> MLNQELELSLNMAFARAREHRHEFMTVEHLLLALLSNPSAREALEACSVDLVALRQELEAFIEQTTPVLPASEEERDTQPTLSFQRVLQRAVFHVQSSGRNE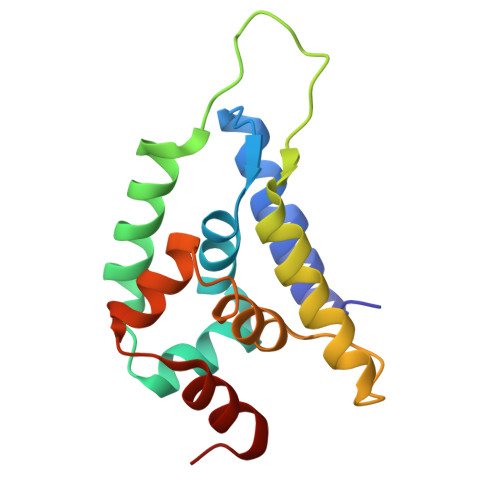VTGANVLVAIFSEQESQAAYLLRKHEVSRLDVVNFISHGT>[2x]GSHMADKELKFLVVDDFSTMRRIVRNLLKELGFNNVEEAEDGVDALNKLQAGGYGFVISDWDMPNMDGLELLKTIRADGAMSALP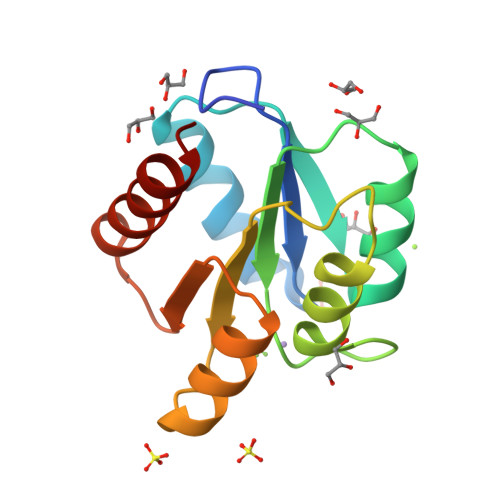VLMVTAKAKKENIIAAAQAGASGYVVKPFTAATLEEKLNKIFEKLGM> PELPEVETIRRTLLPLIVGKTIEDVRIFWPNIIRHPRDSEAFAARMIGQTVRGLERRGKFLKFLLDRDALISHLRMEGRYAVASALEPLEPHTHVVFCFTDGSELRYRDVRKFGTMHVYAK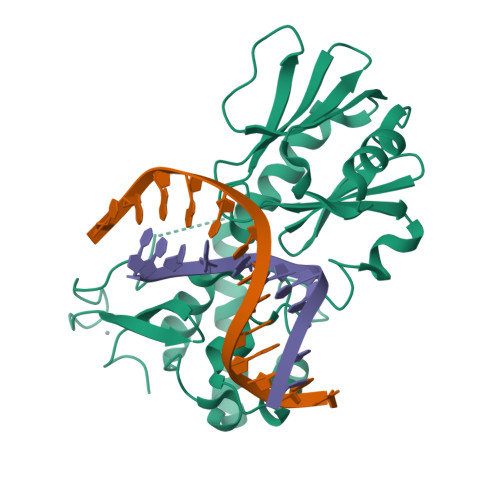EEADRRPPLAELGPEPLSPAFSPAVLAERAVKTKRSVKALLLDCTVVAGFGNIYVDESLFRAGILPGRPAASLSSKEIERLHEEMVATIGEAVMKGGQHHLYVYGRQGNPCKRCGTPIEKTVVAGRGTHYCPRCQR(2S,4S,5S)-5-amino-N-(3-amino-2,2-dimethyl-3-oxopropyl)-4-hydroxy-6-{4-[2-(3-methoxypropoxy)phenyl]-3-oxopiperazin-1-yl}-2-(propan-2-yl)hexanamide 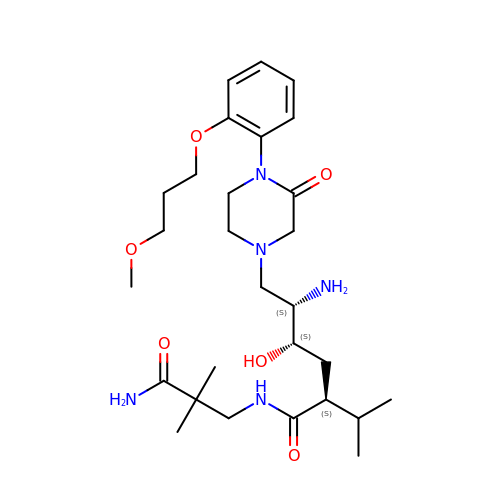| C28 H47 N5 O6 | FOAHAYKWNMPVJI-FUDKSRODSA-N>[4x]MKVGIDAGGTLIKIVQEQDNQRTFKTELTKNIDQVVEWLNQQQIEKLCLTGGNAGVIAENINIPAQIFVEFDAASQGLGILLKEQGHDLADYIFANVGTGTSLHYFDGQSQRRVGGIGTGGGMIQGLGYLLSQITDYKQLTDMAQHGDRNTIDLKVRHIYKDTEPPIPGDLTAANFGHVLHHLDADFTPSNKLAAVI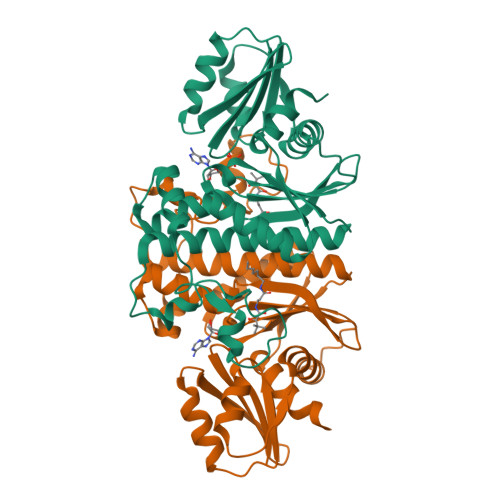GVVGEVVTTMAITVAREFKTENIVYIGSSFHNNALLRKVVEDYTVLRGCKPYYVENGAFSGAIGALYLEK> GCSTPLGMENGKIENKQITASSFKKSWWGDYWEPFRARLNAQGRVNAWQAKANNNKQWLEIDLLKIKKITAIITQGCKSLSSEMYVKSYTIHYSEQGVEWKPYRLKSSMVDKIFEGNTNTKGHVKNFFNPPIISRFIRVIPK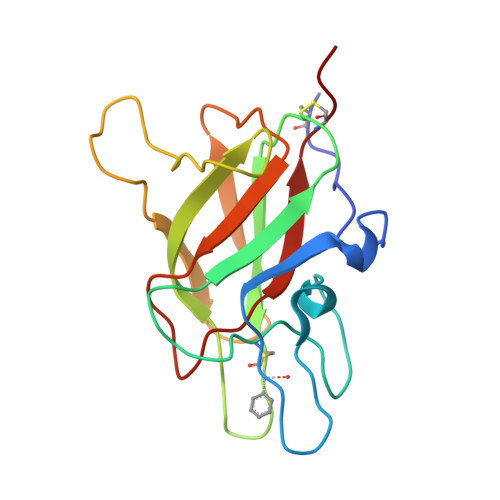TWNQSITLRLELFGCDIY>SNAMAEIKITPEELERI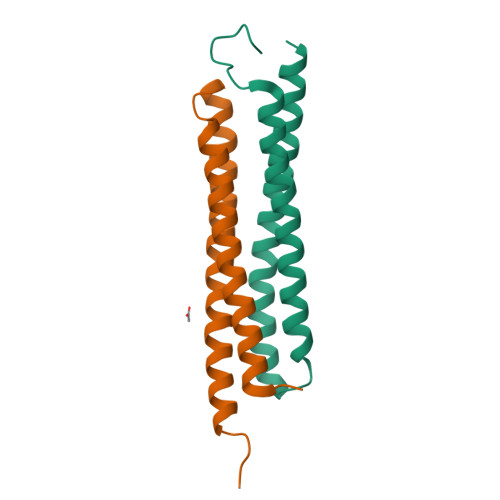AGNFKNAAGEAQSQINRLEGDINSLEGQWAGATQAKFRGEFIQSKQAMQQYIAILEGISTDLKRIADKFRNTDNAY[6x]>MSGSHHHHHHSGSMSERPSDLVVNRLVLFVVKGTATSTNNTVKPLILLEELGVPHDIYVVEKVSAPWFSEINPHKMVPAILDRSPDGRDTLRAWESTSTLMYIADAYDKDGTFGGRNVQERSEINNWLTLHTAALGPTAKYWLYFYKLHPEKLPKTIEKLRSN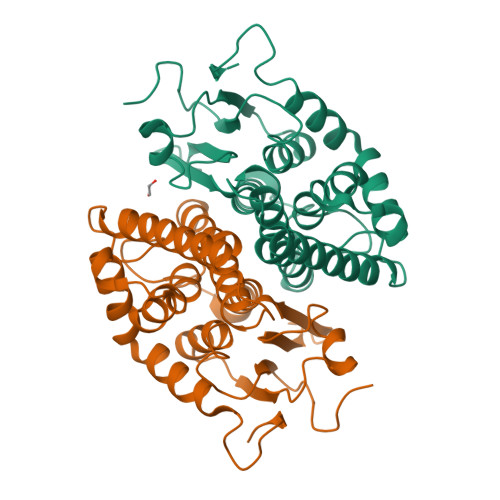ITVQYDILERRLNEPGQQYLALKDRPTIADIATLPFAMKSTAELFGLEFEKWPKLQEWSVRMGEREAVKRAWQRVAGFGHGEKEYGMLEA[6x]>TETTSFSITKFGPDQQNLIFQGDGYTTKERLTLTKAVRNTVGRALYSSPIHIWDSKTGNVANFVTSFTFVIDAPNSYNVADGFTFFIAPVDTKPQTGGGYLGVFNSKDYDKTSQTVAVEFDTFYNTAWDPSNGDRHIGIDVNSIKSINTKSWALQNGKEANVVIAFNAATNVLTVSLTYPN[4x];>[4x]ETSYTLNEVVPLKEFVPEWVRIGFSATT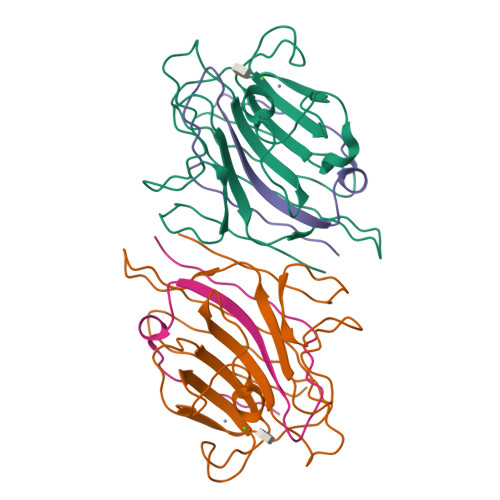GAEFAAHEVLSWYFHSELAGTSSS>[2x]SMAKAKAPRRTLDSYTVKPINKTVKPGDCVLMRPSDPSKPSYVAKIERIESDGRGPNVRVRVRWYYRPEESIGGRRQFHGSKEVFLSDHYDTQSADTIEGKCMVHSFKNYTK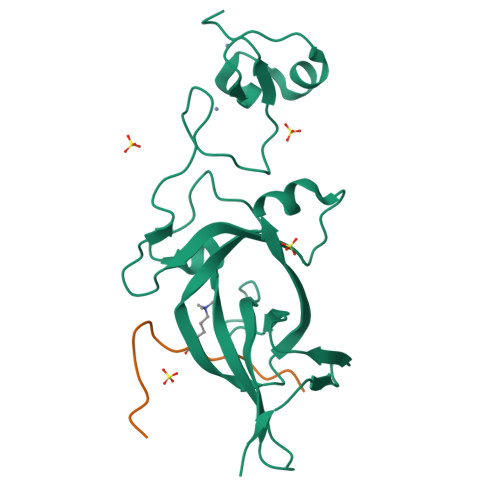LDAVGNDDFFCRFEYNSSTGAFNPDRVAVYCKCEMPYNPDDLMVQCEGCSDWFHPACIEMSAEEAKRLDHFFCENCSSEGQKKLQNSHNTRQSDAKAETKRRRR;>LATKAARKSAPATGGVK[2x]5'-O-[(R)-({5-[(3R)-1,2-DITHIOLAN-3-YL]PENTANOYL}OXY)(HYDROXY)PHOSPHORYL]ADENOSINE 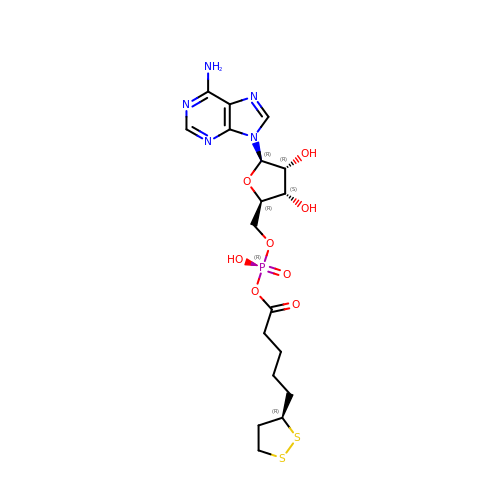| C18 H26 N5 O8 P S2 | QWEGOCJRZOKSOE-ADUAKINBSA-N> MNYNLSKYPDDVSRLFKPRPPLSYKRPTDYPYAKRQTNPNIT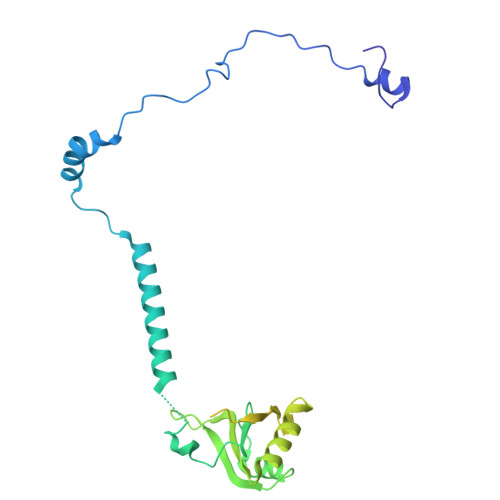GVANLLSTSLKHYMEEFPEGSPNNHLQRYEDIKLSKIKNAQLLDRRLQNWNPNVDPHIKDTDPYRTIFIGRLPYDLDEIELQKYFVKFGEIEKIRIVKDKITQKSKGYAFIVFKDPISSKMAFKEIGVHRGIQIKDRICIVDIERGRTVKYFKPRRLGGGLGGRGYSNRDSRLPGRFASASTSNPAERNYAPRLPRRETSSSAYSADRYGSSTLDARYRGNRPLLSAATPTAAVTSVYKSRNSRTRESQPAPKEAPDY>ADKLPYKVADIGLAAWGRKALDIAENEMPGLMRMREMYSASKPLKGARIAGCLHMTVETAVLIETLVALGAEVRWSSCNIFSTQDHAAAAIAKAGIPVFAWKGETDEEYLWCIEQTLHFKDGPLNMILDDGGDLTNLIHTKHPQLLSGIRGISEETTTGVHNLYKMMANGILKVPAINVNDSVTKSKFDNLYGCRESLIDGIKRATDVMIAGKVAVVAGYGDVGKGCAQALRGFGARVIITEIDPINALQAAMEGYEVTTMDEACKEGNIFVTTTGCVDIILGRHFEQMKDDAIVCNIGHFDVEIDVKWLNENAVEKVNIKPQVDRYLLKNGHRIILLAEGRLVNLGCAMGHPSFVMSNSFTNQVMAQIELWTHPDKY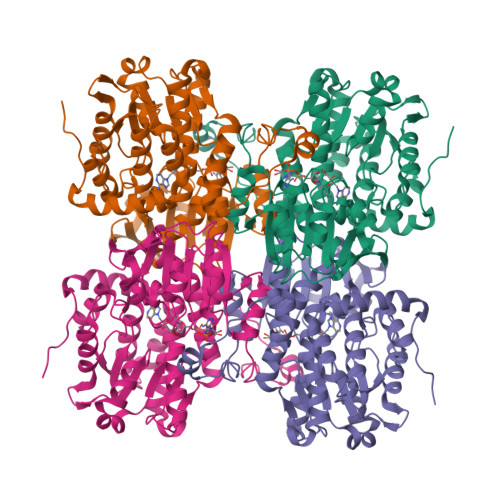PVGVHFLPKKLDEAVAEAHLGKLNVKLTKLTEKQAQYLGMPINGPFKPDHYRY[8x]> MARKYFVAANWKCNGTLESIKSLTNSFNNLDFDPSKLDVVVFPVSVHYDHTRKLLQSKFSTGIQNVSKFGNGSYTGEVSAEIAKDLNIEYVIIGHFERRKYFHETDEDVREKLQASLKNNLKAVVSFGESLEQREQNKTIEVITKQVKAFVDLIDNFDNVILVYEPLWAIGTGKTATPEQAQLVHKEIRKIVKDTCGEKQANQIRILYGGSVNTENC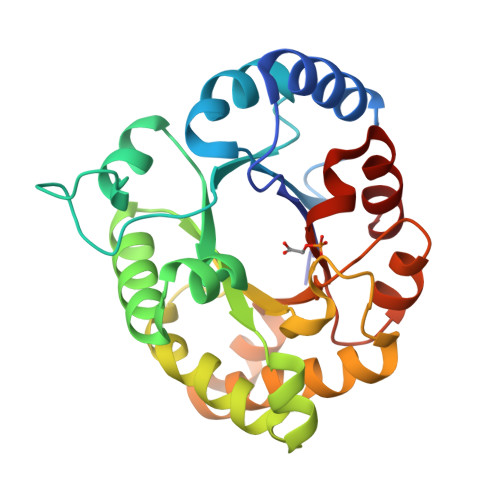SSLIQQEDIDGFLVGNASLKESFVDIIKSAM>[3x]MNSQLTLRALERGDLRFIHNLNNNRNIMSYWFEEPYESFDELEELYNKHIHDNAERRFVVEDAQKNLIGLVELIEINYIHRSAEFQIIIAPEHQGKGFARTLINRALDYSFTILNLHKIYLHVAVENPKAVHLYEECGFVEEGHLVEEAFINGRYQDVKRMYILQSKYLNRSE

Spermidine/spermine N-acetyltransferases (SSATs) are catabolic enzymes that acetylate polyamines and are critical for maintaining intracellular polyamine homeostasis. SpeG is an SSAT protein found in a variety of bacteria, including the human pathogen Vibrio cholerae. This protein adopts a dodecameric structure and contains an allosteric site, making it unique compared to other SSATs. The allosteric site is located between monomers that form the hexamers of the dodecamer, and some evidence has been provided that shows when polyamine binds to these sites, the dodecamer tightens.

Our analysis of the spm-bound structure of VcSpeG showed these two regions form potentially significant contacts: π-π interactions between F32 and F149 and an H-bond between R25 and N152. To elucidate whether these residues could be important for stabilizing the interaction between these two regions of VcSpeG, we created three point mutants: N152L, F149A, and F149G (R3C4-R3C6). We substituted leucine for asparagine at position 152 to retain the overall structural similarity of the residue but remove the ability to H-bond, and we substituted alanine and glycine for phenylalanine at position 149 to potentially decrease the ability of this residue to form hydrophobic interactions. During our kinetic analyses we found the VcSpeG N152L (R3C4), F149A (R3C5), and F149G (R3C6) mutant enzymes still retained reasonably high activity toward spm. The catalytic efficiency of the N152L mutant increased slightly (1.2-fold), and the F149A and F149G mutants decreased 1.4- and 5.3-fold, respectively compared to WT. Our analysis of the spm-bound homology models for the R3C4-R3C6 constructs showed all three retained spm in the allosteric site. On the other hand, when we replaced phenylalanine with alanine (R3C5) and with glycine (R3C6) at position 149, the π-π interactions between F32 and F149 were removed and the H-bond between R25 and N152 side chains remained. In contrast, an alanine substitution at position 149 still has hydrophobic character and may be sufficient for the H-bond between R25 and N152 to be retained as shown in the homology model. The single point mutants we tested in Region 3 (F149, N152; R3C4-R3C6) were insufficient to totally inhibit enzyme activity. In cases where only a single residue in this region was altered (R3C4-R3C6), the disruption to the activity was far less.>[4x]GAMGSMATRIAILGAGPSGMAQLRAFQSAQEKGAEIPELVCFEKQADWGGQWNYTWRTGLDENGEPVHSSMYRYLWSSGPKECLEFADYTFDEHFGKPIASYPPREVLWDYIKGRVEKAGV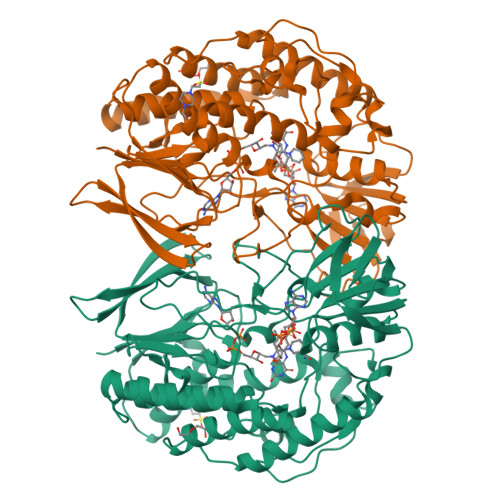RKYIRFNTAVRHVEFNEDSQTFTVTVQDHTTDTIYSAAFDYVVCCTGHFSTPYVPEFEGFEKFGGRILHAHDFRDALEFKDKTVLLVGSSYSAEDIGSQCYKYGAKKLISCYRTAPMGYKWPENWDERPNLVRVDTENAYFADGSSEKVDAIILCTGYIHHFPFLNDDLRLVTNNRLWPLNLYKGVVWEDNPKFFYIGMQDQWYSFNMFDAQAWYARDVIMGRLPLPSKEEMKADSMAWREKELTLVTAEEMYTYQGDYIQNLIDMTDYPSFDIPATNKTFLEWKHHKKENIMTFRDHSYRSLMTGTMAPKHHTPWIDALDDSLEAYLSDKSEIPVAKEA> AIGPVADLTISNGAVSPDGFSRQAILVNDVFPSPLITGNKGDRFQLNVIDNMTNHTMLKSTSIHWHGFFQHGTNWADGPAFVNQCPISTGHAFLYDFQVPDQAGTFWYHSHLSTQYCDGLRGPIVVYDPNDPHASLYDVDDDSTVITLADWYHLAAKVGAPVPTADATLINGLGRSAATLAADLAVITVTKGKRYRFRLVSLSCDPNYTFSIDGHSLTVIEADSVNLKPH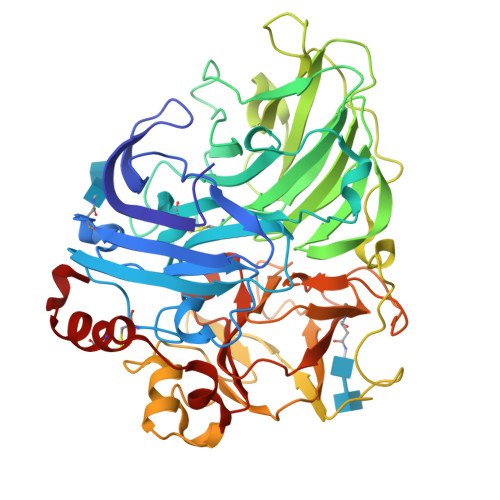TVDSLQIFAAQRYSFVLNADQDVDNYWIRALPNSGTQNFAGGTNSAILRYDGAAPVEPTTSQTPSTNPLVESALTTLKGTAAPGSPTPGGVDLALNMAFGFAGGNFTINGASFTPPTVPVLLQILSGAQSAADLLPAGSVYSLPANADIEISLPATAAAPGFPHPFHLHGHVFAVVRSAGSSTYNYANPVYRDVVSTGAPGDNVTIRFRTDNPGPWFLHCHIDFHLEAGFAVVMAEDIPDVAATNPVPQAWSDLCPTYDALSPDDQ>GGSGPLKPEEHEDILNKLLDPELAQSERTEALQQLRVNYGSFVSEYNDLTKKMDADLSQLQTEVEEAVQECRNAEEKAKKAITDAAMMAEELKKEQDTSAHLERMKKNM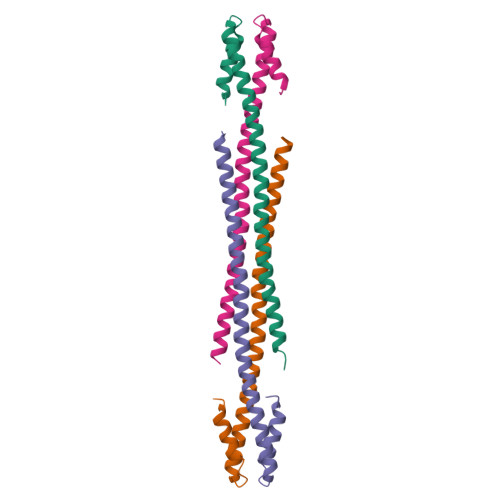[4x]> SGLYVAAKFSESTLDALEELQRSLKLPNP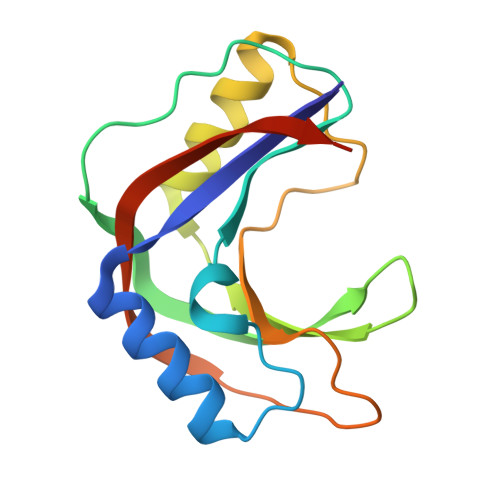VPRDKLHTTIVYSRVNVPYKVASGSFEIADKGKLTVFETQSGNRALVLEMDSDYLSARHSYAKALGASYDYPDYRPHITLSYNIGVLNFSGEYKVPVVLDREYSEELDLEWSDKD> MKKLVKLAAFGAAAAVAATLGAIAPASAHGEKSQQAFLRMRTLNWYDVQWSKTTVNVNEEMILSGKVHVFSAWPQAVANPRVSFLNAGEPGPVLVRTAQFIGEQFAPRSVSLEIGKDYAFSINLRGRRAGRWHVHAQINVEGGGPIIGPGQWIEIKGDMKDFTDPVTLLDGSTVDLENYGISRIYA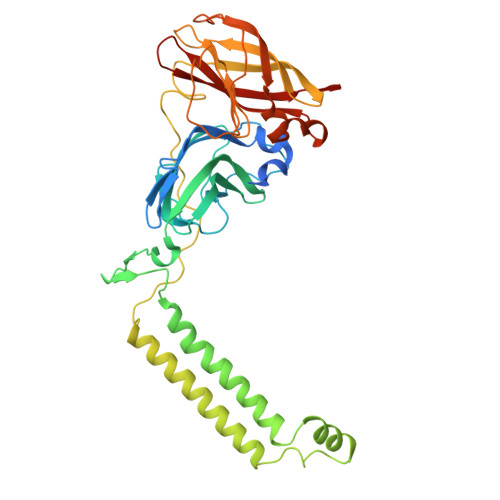WHLPWLAVGAAWILFWFIRKGIIASYVRVAEGRPDDVIGDDDRRIGAIVLALTILATIVGYAVTNSTFPRTIPLQAGLQKPLTPIETEGTVGVGKEQVTTELNGGVYKVPGRELTINVKVKNGTSQPVRLGEYTAAGLRFLNPTVFTQKPDFPDYLLADRGLSNDDVIAPGESKEIVVKIQDARWDIERLSDLAYDTDSQVGGLLFFFTPDGKRFAAEIGGPVIPKFVAGDMP> SPKPTCMVP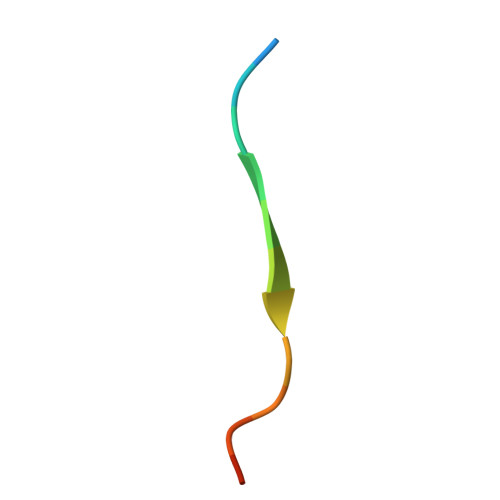PMPHS6-[2-(3-fluoro-5-{2-[(2S)-pyrrolidin-2-yl]ethyl}phenyl)ethyl]-4-methylpyridin-2-amine 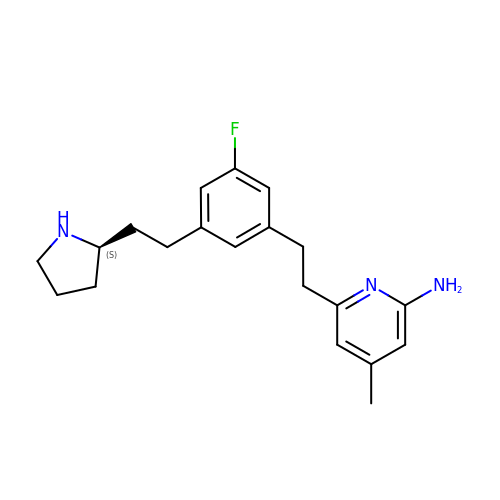| C20 H26 F N3 | PTOVOAJZRWYLQM-GOSISDBHSA-N The cellular retinoic acid-binding proteins CRABPI and CRABPII act as gatekeepers and facilitators for the passage of all-trans-retinoic acid (and related derivatives) through the cytoplasm to access retinoic acid receptors (RARs) in the nucleus. In this article, crystal structures are presented of the L29C mutant of Homo sapiens CRABPI in complex with naturally occurring fatty acids (1.64 Å resolution) and with the synthetic retinoid DC645 (2.41 Å resolution), and of CRABPII in complex with the ligands DC479 (1.80 Å resolution) and DC645 (1.71 Å resolution). The retinoic acid-binding ability of both CRABPI and CRABPII is centred on a hydrophobic pocket created by an orthogonal β-sheet fold and capped with a pair of antiparallel α-helices formed from residues 15–35 partway into the sequence. The pocket contains, at its most buried end, a trio of residues (Arg112, Arg132 and Tyr134 in CRABPI; Arg112, Arg133 and Tyr135 in CRABPII) that are responsible for binding to the carboxylic acid moiety of ATRA, usually in concert with a water molecule that is conserved in all structures with similarly binding ligands.

As part of crystal-screening efforts, we identified that an L29C mutation in Homo sapiens CRABPI allowed vastly improved crystallization and diffraction to atomic resolution, which was subsequently determined to be due to partial dimerization at the mutated surface residue. This mutation is found on the outer edge of the cap helices and as such does not affect the make-up of the hydrophobic binding site. The crystal structure resulting from molecular replacement contained unknown density in the ligand-binding sites of both independent monomers that was not suitable for fitting either ATRA or the synthetic ligands used for co-crystallization. It was determined that this density was most likely to represent fatty-acid byproducts from expression that were incorporated into the binding site based on their hydrophobic structure and carboxylic acid head group, and it was therefore fitted as the 14-carbon myristic acid (MYR) and the 13-carbon tridecanoic acid (TDA) in the two monomers. CRABPI shares high sequence similarity with other members of the fatty acid-binding protein family and so the incorporation of MYR/TDA molecules is a logical step for a protein produced recombinantly in E. coli in the absence of its natural ligand. Similarly, it has been shown that RXRs and other retinoid-binding proteins treat fatty acids (including myristic acid) as ligands, and so it is possible that nongenomic pathways are similarly influenced. To date, CRABPI had only been crystallized using the proteins from M. musculus and B. taurus. Whilst they are nearly identical, H. sapiens CRABPI contains a single amino-acid shift from alanine to proline at position 86.

>[2x]MPNFAGTWKMRSSENFDELLKALGVNAMCRKVAVAAASKPHVEIRQDGDQFYIKTSTTVRTTEINFKVGEGFEEETVDGRKCRSLATWENENKIHCTQTLLEGDGPKTYWTRELANDELILTFGADDVVCTRIYVRE3-(2-chlorophenyl)-6-(1,3-dimethyl-5-oxidanyl-pyrazol-4-yl)carbonyl-1,5-dimethyl-quinazoline-2,4-dione | C22 H19 Cl N4 O4 | 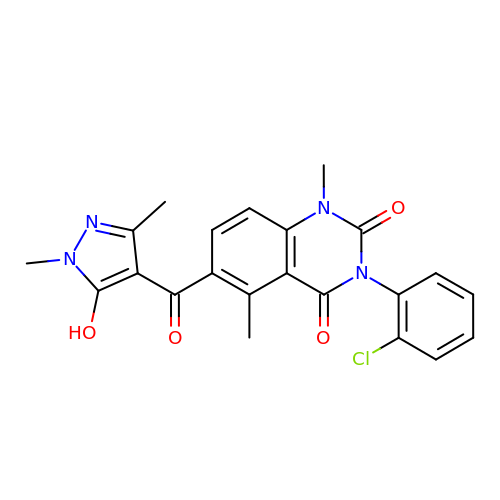TUTSWQSDTDEPDU-UHFFFAOYSA-N N-[(S)-hydroxy(4-phenylbutoxy)phosphoryl]-L-glutamic acid 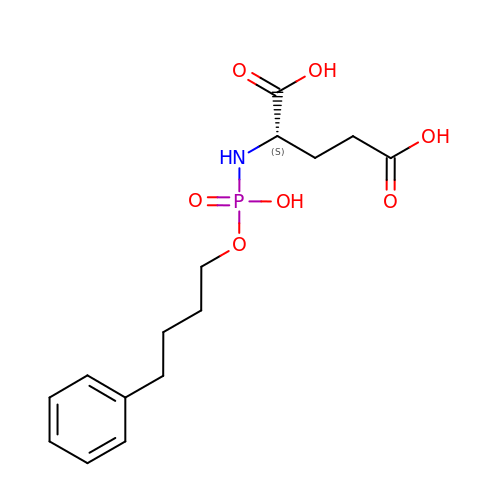| C15 H22 N O7 P | QQDXXPMQJXSLMC-ZDUSSCGKSA-N>[4x]LRNATQRMFEIDYSRDSFLKDGQPFRYISGSIHYSRVPRFYWKDRLLKMKMAGLNAIQTYVPWNFHEPWPGQYQFSEDHDVEYFLRLAHELGLLVILRPGPYICAEWEMGGLPAWLLEKESILLRSSDPDYLAAVDKWLGVLLPKMKPLLYQNGGPVITVQVENEYGSYFACDFDYLRFLQKRFRHHLGDDVVLFTTDGAHKTFLKCGALQGLYTTVDFGTGSNITDAFLSQRKCEPKGPLINSEFYTGWLDH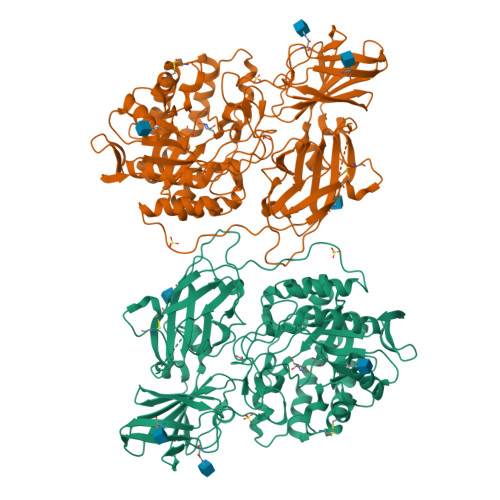WGQPHSTIKTEAVASSLYDILARGASVNLYMFIGGTNFAYWNGANSPYAAQPTSYDYDAPLSEAGDLTEKYFALRNIIQKFEKVPEGPIPPSTPKFAYGKVTLEKLKTVGAALDILCPSGPIKSLYPLTFIQVKQHYGFVLYRTTLPQDCSNPAPLSSPLNGVHDRAYVAVDGIPQGVLERNNVITLNITGKAGATLDLLVENMGRVNYGAYINDFKGLVSNLTLSSNILTDWTIFPLDTEDAVRSHLGGWGHRDSGHHDEAWAHNSSNYTLPAFYMGNFSIPSGIPDLPQDTFIQFPGWTKGQVWINGFNLGRYWPARGPQLTLFVPQHILMTSAPNTITVLELEWAPCSSDDPELCAVTFVDRPVIGSSVTYDHPSKPVEKRLMPPPPQKNKDSWLDHV> MAVTSESVPEQQITAYLLKIQRGGFIQPFGSMIAVDEPSFRILAYSDNARDMLGITPQSVPSLDDKNDAAFALGTDIRTLFTHSSAVLLEKAFSAREISLMN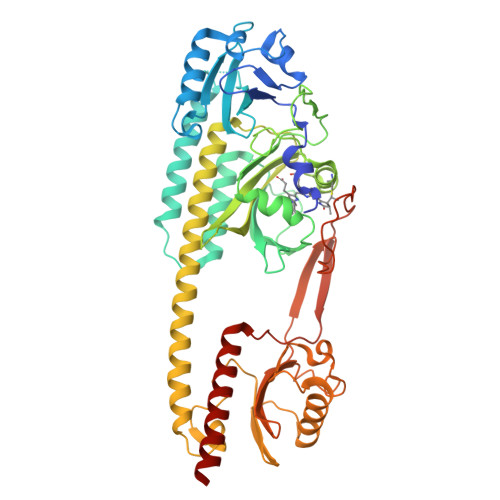PIWIHSRTSGKPFYGILHRIDVGIVIDLEPARTEDPALSIAGAVQSQKLAVRAISQLQSLPGGDVKLLCDTVVESVRELTGYDRVMVYRFHEDEHGEVVAETKRPDLEPYIGLHYPATDIPQASRFLFKQNRVRMIVDCHASAVRVVQDEALVQPLCLVGSTLRAPHGCHAQYMANMGSTASLVMAVIINGNDEEGVGGRTSMRLWGLVVCHHTSARCIPFPLRYACEFLMQAFGLQLNMELQLAAQSLEKRVLRTQTLLCDMLLRDSPTGIVTQSPSIMDLVKCDGAALYYQGNYYPLGVTPTEAQIRDIIEWLLAFHRDSTGLSTDSLADAGYPGAASLGDAVCGMAVAYITEKDFLFWFRSHTAKEIKWGGAKHHPEDKDDGQRMHPRSSFKAFLEVVKSRSLPWENAEMDAIHSLQLILRDSFKDAEHHHHHH>[2x]MEKFLVIAGPCAIESEELLLKVGEEIKRLSEKFKEVEFVFKSSFDKANRSSIHSFRGHGLEYGVKALRKVKEEFGLKITTDIHESWQAEPVAEVADIIQIPAFLCRQTDLLLAAAKTGRAVNVKKGQFLAPWDTKNVVEKL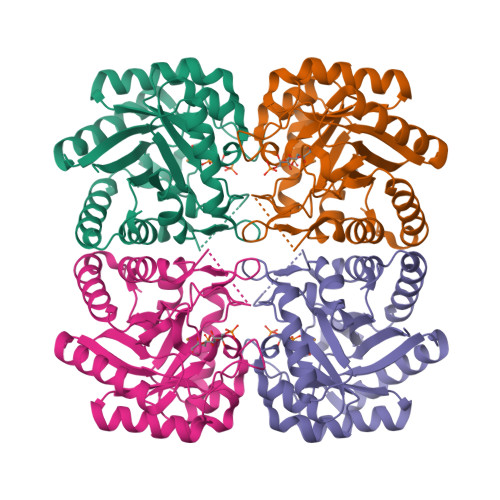KFGGAKEIYLTERGTTFGYNNLVVDFRSLPIMKQWAKVIYDATHSVQLPGGLGDKSGGMREFIFPLIRAAVAVGCDGVFMETHPEPEKALSDASTQLPLSQLEGIIEAILEIREVASKYYETIPVK>QVEGRKAWIIGSGIAGLASAFYLIRDGRMKGQDITILDAVGTPGGSLDGSGNAEDGYLIRGGREMNWNYDHFWDLFQDIPALEYPSPYSVLDEYRAVNDNDPNWSKSRLMHKQGQIRDFSTLGLSSAHQWELIKLLLKRKEDLDDITIEQYFSD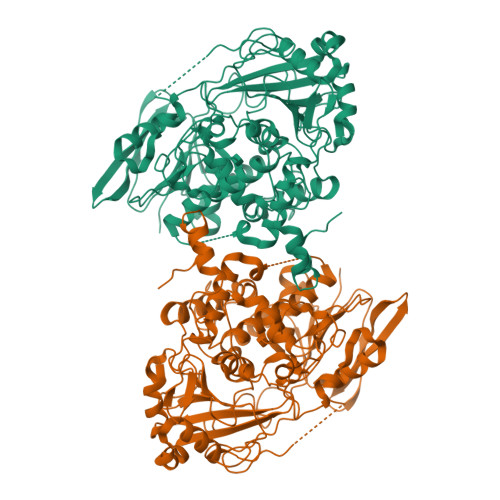SFLETNFWYLWRSMFAFQNWQSLLEVKLYMHRFLDAIDGLTDMSALVFPKYNQYDSFVVPLVNYLKGQGVNVEFGTRVYDLDMTDNNGERTVTSILAKVDGRDQKIDIGAKDVVFALTGSMTEGTAYGDLDTAPDLTRATTPPGDSSDWALWQNLAKKSHVFGKPEKFCGQPSRSMWESATLTCKPSPLTERLKDLSINDPYSGKTVTGGIITFTDSNWVLSFTCNRQPHFPTQPDDVLVLWVYALVMDSKGNHVLKPMPECTGREILAELCYHLGIVDQVDEVARQTKVRLALMPFITAQFMPRAAGDRPRVVPAGCTNLALLGQFVETSNDIIFTMESSVRTARIGVYTLLGLRKQVADISPTQYDVRNLIKGARALNNNEPFMGERLLHRLLDNTYFAHILPPLPAGDGGSSDQAASSRMKANHTAAAALGAVSDWIHHVRDKLKPGA[2x]>[4x]MVKEFNTQTELSVRLEALWAVLSKDFITVVPKVLPHIVKDVQLIEGDGGVGTILIFNFLPEVSPSYQRE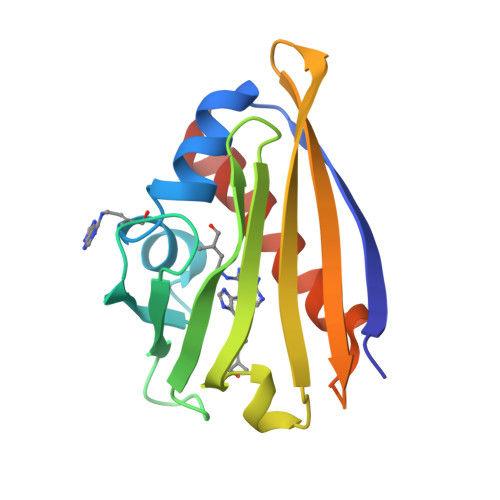EITEFDESSHEIGLQVIEGGYLSQGLSYYKTTFKLSEIEEDKTLVNVKISYDHDSDIEEKVTPTKTSQSTLMYLRRLERYLSNGSA> MEDYDYVH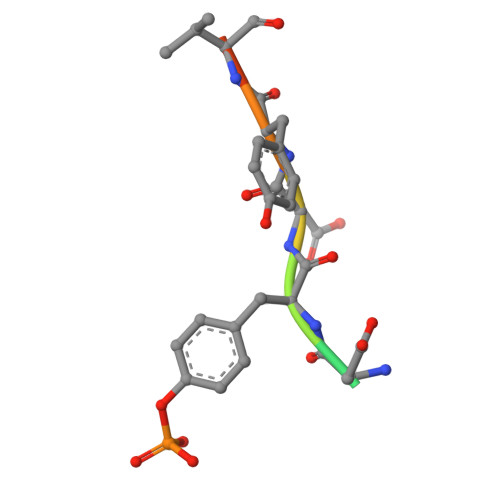L>[2x]MTALTAQVALVTGASRGIGKATALALAATGMKVVVNYAQSSTAADAVVAEIIA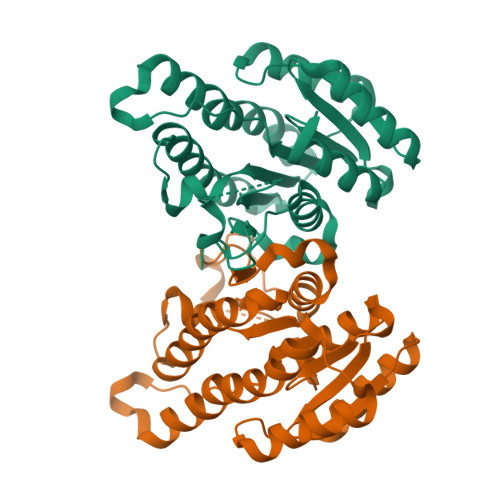NGGEAIAVQANVANADEVDQLIKTTLDKFSRIDVLVNNAGITRDTLLLRMKLEDWQAVIDLNLTGVFLCTKAVSKLMLKQKSGRIINITSVAGMMGNPGQANYSAAKAGVIGFTKTVAKELASRGVTVNAVAPGFIATDMTENLNAEPILQFIPLARYGQPEEVAGTIRFLATDPAAAYITGQTFNVDGGMVMF N-(MORPHOLIN-4-YLSULFONYL)-L-PHENYLALANYL-3-(2-AMINO-1,3-THIAZOL-4-YL)-N-{(1R,2R,3S)-1-[(1R)-CYCLOHEX-3-EN-1-YLMETHYL]-2,3-DIHYDROXY-5-METHYLHEXYL}-L-ALANINAMIDE 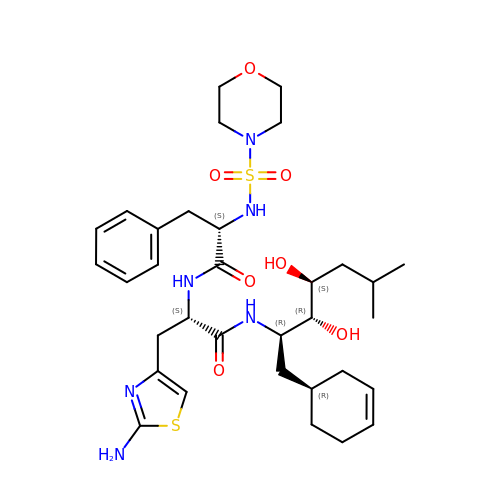| C33 H50 N6 O7 S2 | NZCOCZHRRKSGSQ-LUFJSDQJSA-N>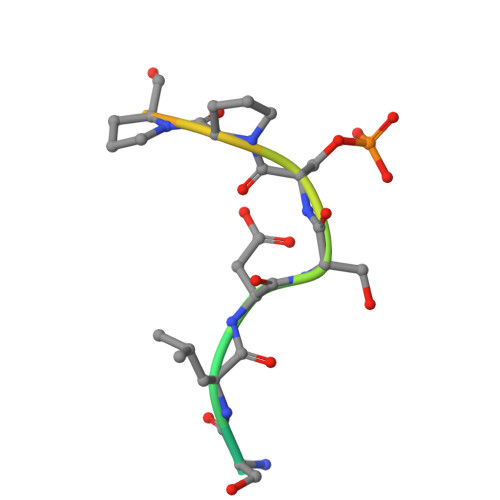 ESPPSLDSSPPNTSFNA>[2x]HMAVKKIAIFGATGQTGLTTLAQAVQAGYEVTVLVRDSSRLPSEGPRPAHVVVGDVLQAADVDKTVAGQDAVIVLLGTRNDLSPTTVMSEGARNIVAAMKAHGVDKVVACT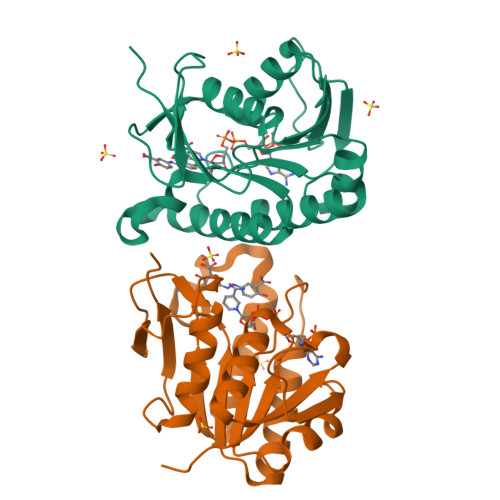SAFLLWDPTKVPPRLQAVTDDHIRMHKVLRESGLKYVAVMPPHIGDQPLTGAYTVTLDGRGPSRVISKHDLGHFMLRCLTTDEYDGHSTYPSHQYQ>[6x]GVGGVKLENILTIFVQR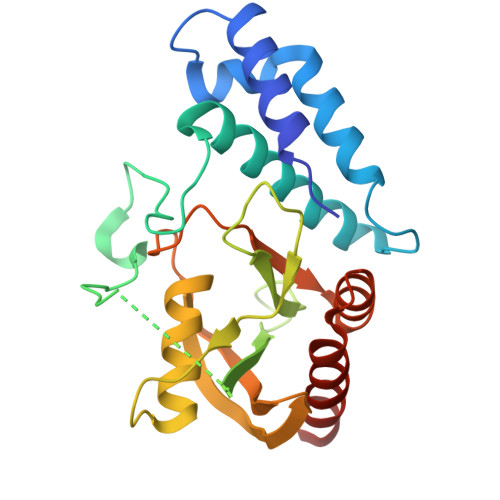AKAKLPQGFTAAALGNWKGFSRRVDTVMEHYPKGLSEKAIKELRTAETKRFTDYAMLGPSDKYNLLRPMQGVDEAMIAPNLVSLTGRKNQVLGDAGGRSVVCNVVMRSEAEGGGILLISSSKLDKQDFILPKGGLEKGEIAYGAAKREVLEEGGVKVKKLKELGVTLVGDKTYESFLMRSKKVYEQWSESRRLRVWLPWDDAILLLKANKHDEMVEIVKQARAAAAAKAA> MENTENSVASKSIKNLEPKI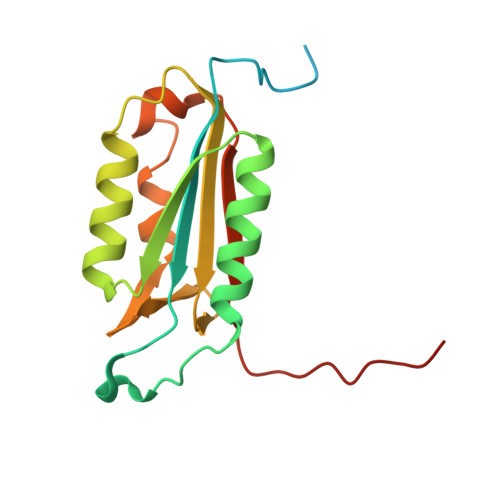IHGSESMASGISLDNSYKMDYPEMGLCIIINNKNFHKSTGMTSRSGTDVDAANLRETFRNLKYEVRNKNDLTREEIVELMRDVSKEDHSKRSSFVCVLLSHGEEGIIFGTNGPVDLKKITNFFRGDRCRSLTGKPKLFIIQACRGTELDCGIETD> MLSHPPIPIADMAEHTERLKANDSLKLSQEYESIDPGQQFTWEHSNLEVNKPKNRYANVIAY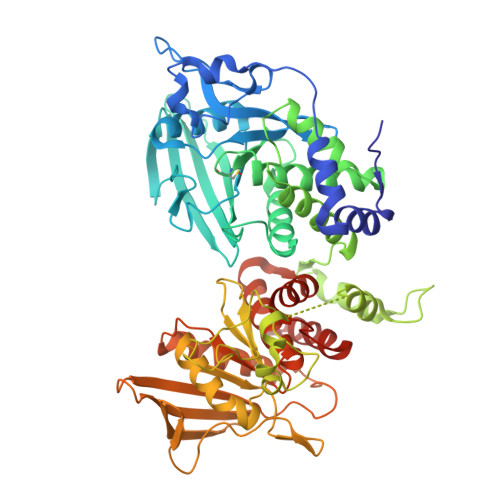DHSRVILQPIEGIMGSDYINANYVDGYRRQNAYIATQGPLPETFGDFWRMVWEQRSATIVMMTRLEEKSRIKCDQYWPNRGTETYGFIQVTLLDTIELATFAVRTFSLHKNGSSEKREVRQFQFTAWPDHGVPEYPTPFLAFLRRVKTANPPDAGPIVVHCSAGVGRTGAFIVIDAMLERIKPEKTVDVYGHVTLMRSQRNYMVQTEDQYSFIHEALLEAVGAGNTEVPARSLYAYIQKLAQVEPGEHVTGMELEFKRLANSKAHTSRFISANLPANKFKNRLVNIMPYESTRVALQPIRGVEGSDYINASFIDGYRQQKAYIATQGPLAETTEDFWRMLWENNSTIVVMLTKLREMGREKCHQYWPAERSARYQYFVVDPMAEYNMPQYILREFKVTDARDGQSRTVRQFQFTDWPEQGVPKSGEGFIDFIGQVHKTKEQFGQDGPISVHCSAGVGRTGVFITLSIVLERMRYEGVVDIFQTVKMLRTQRPAMVQTEDEYQFAYQAALEYLGSFDHYAT> 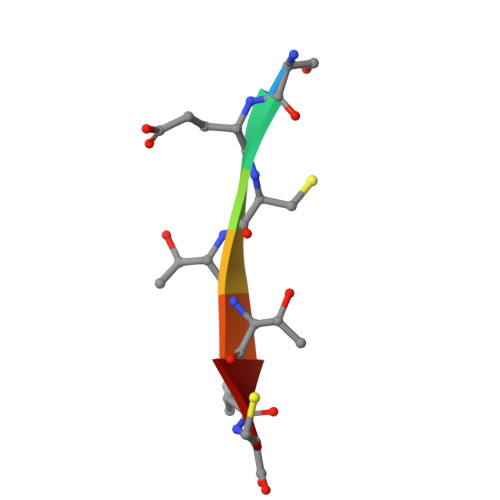SECTTPC>MAFQNDAKANFPDYANHGCVVGRHLNFEMYQRLFGKKTAHGVTVDKVIQPSVDNFGNCIGLIAGDEESYEVFKELFDAVINEKHKGFGPNDSQPAPDLDASKLVGGQFDEKYVKSCRIRTGRGIRGLCYPPSCTRGERREVERVITTALAGLSGDLSGTYYPLSKMTPEQENQLIADHFLFQKPTGHLMVNSASVRDWPDARGIWHNNEKTFLIWINEEDHMRVISMQKGGNVKAVFERFGRGLNAIAEQMKKNGREYMWNQRLGYLCACPSNLGTGLRAS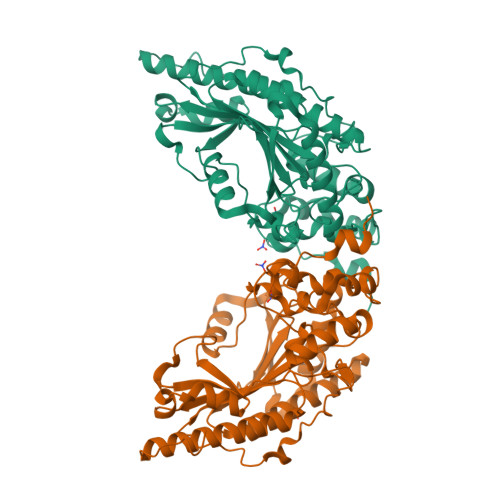VHVQLHQLSKHPKFEDIVVALQLQKRGTGGEHTAAVDDVYDISNAARLKKSEREFVQLLIDGVKKLIDMEQALEAGKSIDDLIPA[2x]> MSAAAAIERRHVAVLDSTMSYVETGASDGPTVLFLHGNPTSSYIWRNIIPHVAPLGRCIAPDLIGFGQSGKPDIDYRFFDHVRYLDAFIDALGIQDVVLVAQDWGTALAFH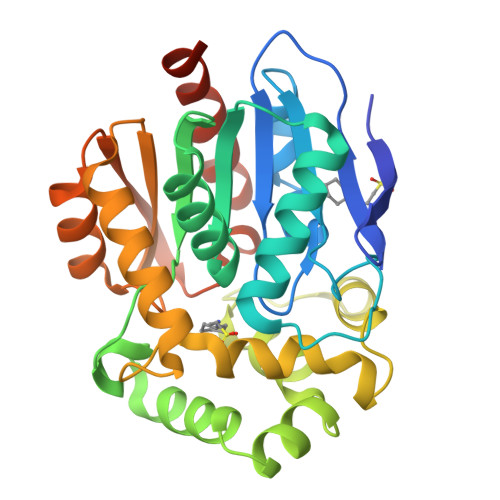LAARRPDRVRGLAFMEFIRPMPTWDDFHQRPQAREMFKAFRTPGVGEKMILEDNVFVEKVLPGSVLRTLSEEEMAVYRAPFPTPESRKPVLRFPRELPIEGEPADVAAILESAHRALAASTYPKLLFAGDPGALISPQAAERFAANLKNCRLINLGPGLHYLQEDHPDAIGRTIAGWLPEIAAASRTAEAHHHHHH>MAHHHHHHMGLLEQRVALVTGAGGGIGRGVARSFGNEGAAVIIAEINESTGRQVEQEIREMGGRSLFVKTDVTSKASIEAAVRSAVEQFGSLDILVNNAFVPTPNVLLEEKTDEMLEQTLTTSLWATWWAMRAAFVPMRERRWGRIVNFYSIDTETGAWLHGDYNTAKAGIVGLTRSAASEWGRFNITVNAIAPTAMGATFFELAAKNPEFAERSAAARPLGRSGDPEQDIGPAAVFFASEMSRFVTGETLHVDGGLHLPGYN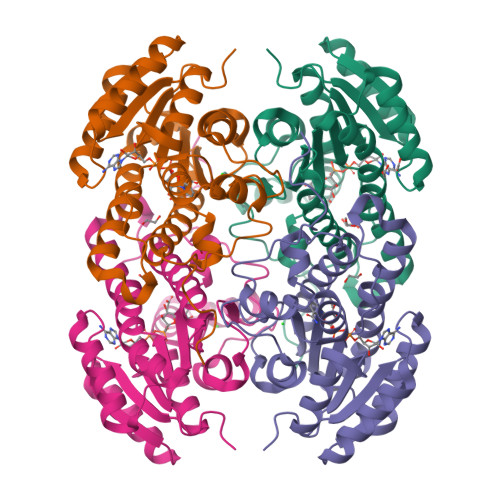SRPAGIKPREY[4x]> EEKEMKPACIKALTRIFKISDQDNDGTLNDAELNFFQRICFNTPLAPQALEDVKNVVRKHISDGVADSGLTLKGFLFLHTLFIQRGRHETTWTVLRRFGYDDDLDLTPEYLFPLLKIPPDCTTELNHHAYLFLQSTFDKHDLDRDCALSPDELKDLFKVFPYIPWGPDVNNTVCTNERGWITYQGFLSQWTLTTYLDVQRCLEYLGYLGYSILTEQESQASAVTVTRDKKIDLQKKQTQRNVFRCNVIGVKNCGKSGVLQALLGRNLMRQKKIREDHKSYYAINTVYVYGQEKYLLLHDISESEFLTEAEIICDVVCLVYDVSNPKSFEYCARIFKQHFMDSRIPCLIVAAKSDLHEVKQEYSISPTDFCRKHKMPPPQAFTCNTADAPSKDIFVKLTTMAMYPHVTQADLKSSTFLEHHHHHH

Human Miro1 and Miro2 (hMiro1, hMiro2, also called RhoT1 and RhoT2) are MOM protein homologs that play a critical role in mitochondrial trafficking38394041424344. Both associate with Parkin upon mitochondrial depolarization and are ubiquitinated on multiple lysines18374546. Here, we demonstrate that the cGTPase domain is necessary and sufficient for efficient ubiquitination of either hMiro1 or hMiro2 by p-S65 Parkin. We also find that despite considerable similarities between these two substrates, Parkin modifies hMiro1 much more robustly than hMiro2.

We determined the crystal structure of hMiro1 amino acids (aa) 177–592 (hMiro1-BC), encompassing the central EF hand region and cGTPase domain, to 2.5 Å resolution. Similarly, structures of hMiro1-BC bound to either GDP or the non-hydrolyzable GTP analog GMPPCP were virtually superimposable, with GTPase Switch 1 positioned far from the nucleotide-binding pocket in both cases. Thus, the structure of hMiro1-BC is highly evolutionarily conserved and, in isolation, appears to be conformationally inert with respect to ion or nucleotide binding. We tested whether different ion or nucleotide conditions might influence Miro ubiquitination efficiency by p-S65 Parkin. Using ion or nucleotide exchange protocols similar to those used to obtain crystal structures of hMiro1 constructs in different divalent cation and nucleotide states, we were unable to detect a change in hMiro1 or hMiro2 ubiquitination. This result suggests that neither the divalent cations Mg2+ and Ca2+ nor the nucleotide ligands GDP and GTP directly regulate Parkin-mediated Miro ubiquitination.2-[[3,5-bis(fluoranyl)-4-oxidanyl-phenyl]amino]-5,7,7-trimethyl-8-(3-methylbutyl)pteridin-6-one 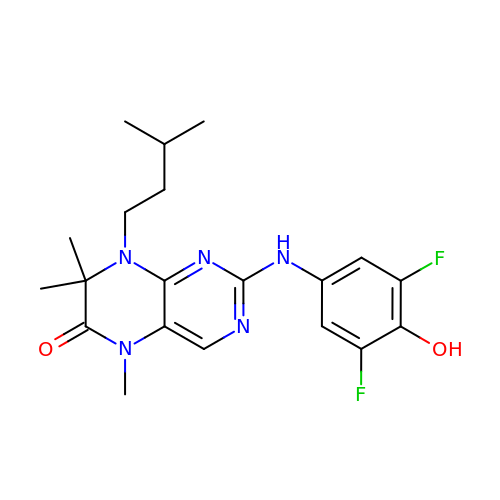| C20 H25 F2 N5 O2 | OBURZOUEBBWMPC-UHFFFAOYSA-N> MGHHHHH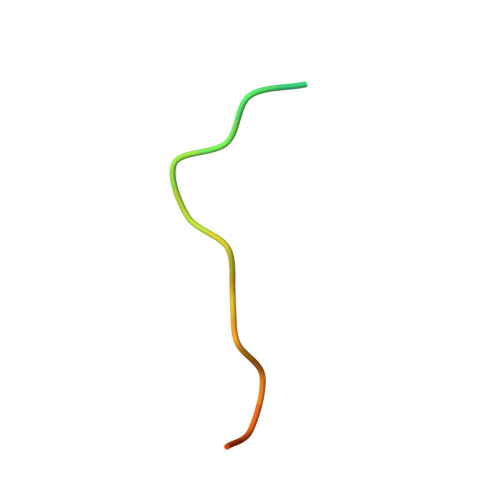HHHHHSSGHIEGRH> MD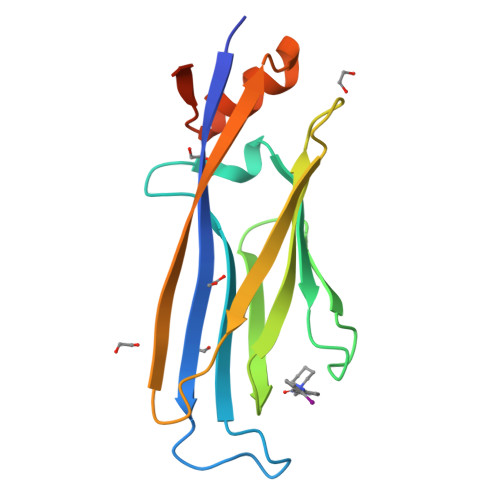NQCTVQVRLELGHRAQLRKKPTTEGFTHDWMVFVRGPEQCDIQHFVEKVVFWLHDSFPKPRRVCKEPPYKVEESGYAGFIMPIEVHFKNKEEPRKVCFTYDLFLNLEGKVNHLRCEKLTFNNPTTEFRYKLLRAGGVMVMPEGAHHHHHH>[3x]QQRRDGKQICEEKARERQQEEGNSSEESYGKEQEENPYVFQDEHFESRVKTEEGRVQVLENFTKRSRLLSGIENFRLAILEANPHTFISPAHFDAELVLFVAKGRATITMVREEKRESFNVEHGDIIRIPAGTPVYMINRDENEKLFIVKILQPVSAPGHFEAFYGAGGEDPESFYRAFSWEVLEAALKVRREQLEKVFGEQSKGSIVKA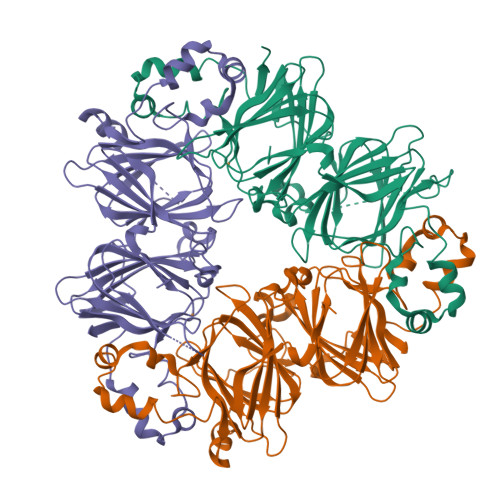SREKIRALSQHEEGPPRIWPFGGESSGPINLLHKHPSQSNQFGRLYEAHPDDHKQLQDLDLMVSFANITKGSMAGPYYNSRATKISVVVEGEGFFEMACPHLSSSSGSYQKISARLRRGVVFVAPAGHPVAVIASQNNNLQVLCFEVNAHGNSRFPLAGKGNIVNEFERDAKELAFNLPSREVERIFKNQDQAFFFPGPNKQQEEGGRGGRAFE>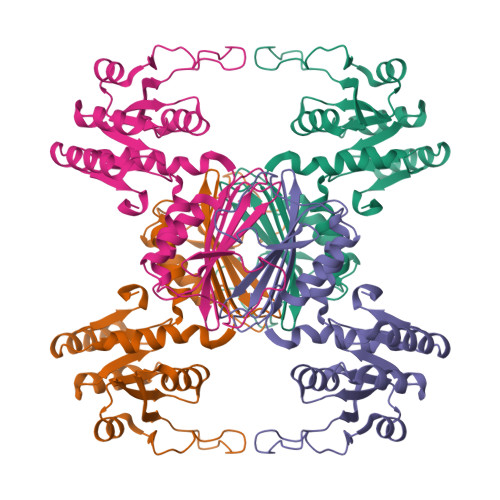 MIRVAIGGPRGKMGQEAVHTVMNNENMELVAVLDHKDIGDLLSESPNFPASYEVPVFLNLESLIVTIKPDVFLDLTTPHQVFEHTMLCLQNNVRPVIGTTGFTDEQLQQCTILAEVNKLGCIVAPNFAIGAVLMMKFASLAAAYFPDVEIIEMHHDQKLDAPSGTAYKTAQMIAEVRPSHKQGHPNEKETLEGARGASYDGIPIHSVRLPGLIAHQQILFGGEGQLFTLRHDSYNRQSFMSGVTFSINQVMEIKELVYGLENIL(2S)-2-[(3aR,4R,7S,7aS)-1,3-dioxooctahydro-2H-4,7-methanoisoindol-2-yl]propanoic acid | C12 H15 N O4 | 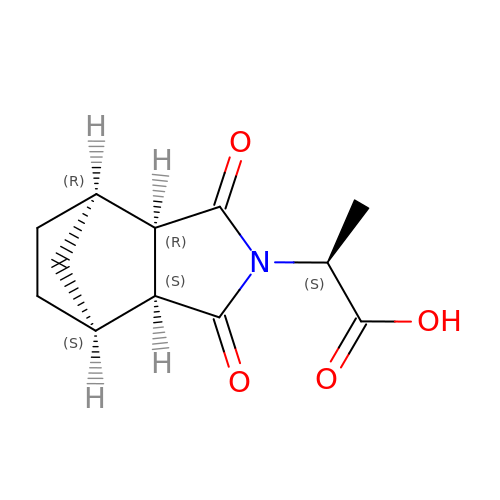REFMTLIXGKZVDF-VRGHQRLXSA-N> IVGGTNSSWGEWPWQVSLQVKLTAQRHLCGGSLIGHQWVLTAAHCFDGLPLQDVWRIYSGILNLSDITKDTPFSQIKEIIIHQNYK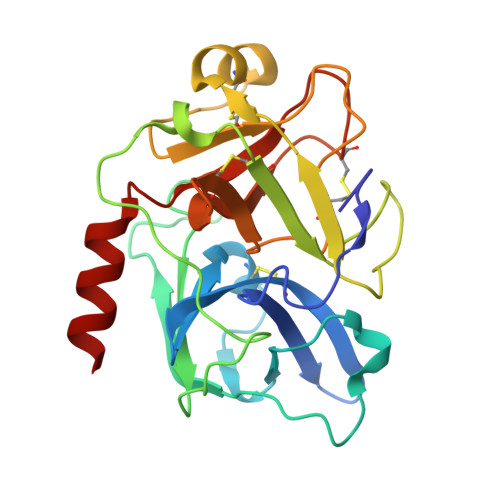VSEGNHDIALIKLQAPLNYTEFQKPISLPSKGDTSTIYTNCWVTGWGFSKEKGEIQNILQKVNIPLVTNEECQKRYQDYKITQRMVCAGYKEGGKDACKGDSGGPLVCKHNGMWRLVGITSWGEGCARREQPGVYTKVAEYMDWILEKTQSSD> KPRIPVVWIHGLECTCCTESFIRSAHPLAKDVILSLISLDYDDTLMAAAGTQAEEVFEDIITQYNGKYILAVEGNPPLGEQGMFCISSGRPFIEKLKRAAAGA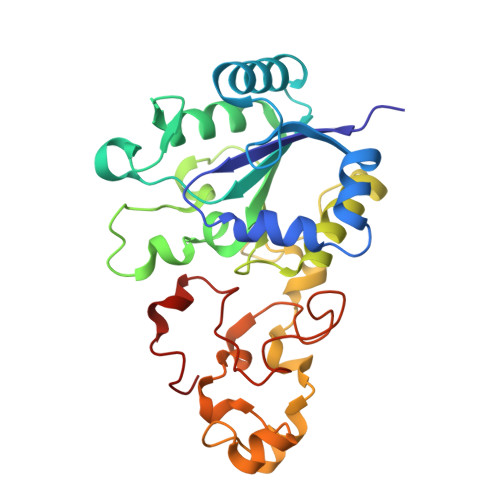SAIIAWGTCASWGCVQAARPNPTQATPIDKVITDKPIIKVPGCPPIPDVMSAIITYMVTFDRLPDVDRMGRPLMFYGQRIHDKCYRRAHFDAGEFVQSWDDDAARKGYCLYKMGCKGPTTYNACSSTRWNDGVSFPIQSGHGCLGCAENGFWDRGSFYSRV> MAKIDNAVLPEGSLVLVTGANGFVASHVVEQLLEHGYKVRGTARSASKLANLQKRWDAKYPGRFETAVVEDMLKQGAYDEVIKGAAGVAHIASVVSFSNKYDEVVTPAIGGTLNALRAAAATPSVKRFVLTSSTVSALIPKPNVEGIYLDEKSWNLESIDKAKTLPESDPQKSLWVYAASKTEAELAAWKFM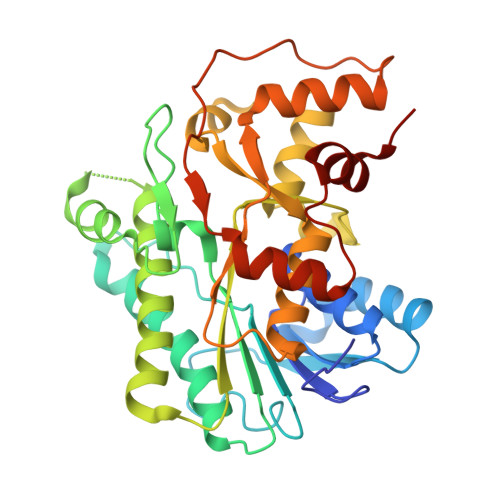DENKPHFTLNAVLPNYTIGTIFDPETQSGSTSGWMMSLFNGEVSPALALFPPTYYVSAVDIGLLHLGCLVLPQIERRRVYGTAGTFDWNTVLATFRKLYPSKTFPADFPDQGQDLSKFDTAPSLEILKSLGRPGWRSIEESIKDLVGSETA> MSNMEKHLFNLKFAAKELSRSAKKCD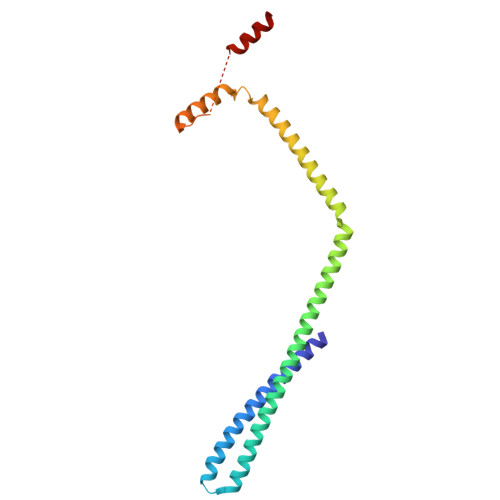KEEKAEKAKIEKAIQKGNMEVARIHAENAIRQKNQAVNFLRMSARVDAVAARVQTAVTMGKVTKSMAGVVKSMDATLKTMNLEKISALMDKFEHQFETLDVQTQQMEDTMSSTTTLTTPQNQVDMLLQEMADEAGLDLNMELPQGQTGSVGTSVASAEQDELSQRLARLRDQV> MSRRPTLRLGLDRDVYNIVLNLEQQGTDENGKRPRLTVDYVYDTIKRSNSSLARQKKRMLEDSIERVLAVRKEQAKAEEETDSDDLIEAQERERERQKAAQAQRDANLLNR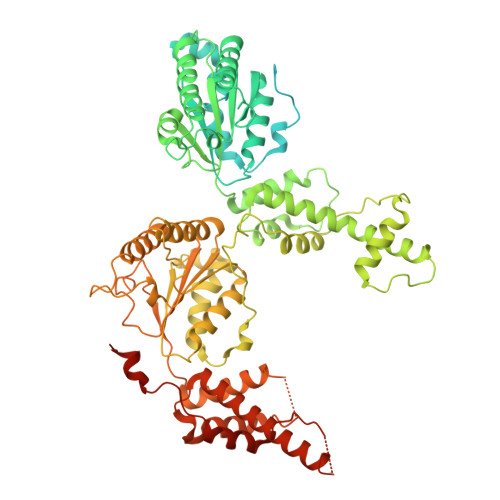QIAKSWGFASSPGAKAADGEKGTDTGSIATPAPATPAVAENMAADTPTTSTGPVLPASSTDRQPNGEPRPKKRKAAPKEIDRTPPTKVSILDIAGVDDTLQRLLKEVWFPLRGGEACEKMGYRYDNGVLLHGPSGCGKTTLAHAIAGSIGVAFIPVSAPSVIGGTSGESEKNIRDVFDEAIRLAPCLIFLDEIDAIAGRRESANKGMESRIVAEIMNGMDRIRQNTPLGKNVVVLAATNRPEFLDPAIRRRFSVEIDMGMPSERAREQILRSLTRDLSLADDINFKELAKMTPGYVGSDLQYVVKAAVSESFQANIDSLLAQARAKHPADHLANVSQPQRDWLLLEAHRDEEVSWPSTKITMEQFRKAVSLVQPASKREGFSTIPDTTWSHVGALEDVRKKLEMSIIGPIKNPELFTRVGIKPAAGILLWGPPGCGKTLVAKAVANESKANFISIKGPELLNKYVGESERAVRQLFSRAKSSAPCILFFDQMDALVPRRDDSLSDASARVVNTLLTELDGVGDRSGIYVIGATNRPDMIDEAIRRPGRLGTSIYVGLPSAEDRVKILKTLYRNTVKAPKKREGTNGEDVDMTDAAAEQQHQGTTDADLEKVALDLRCTGFSGADLGNLMQAAAQACLERVYTQRQQKRKEGGSVAEEEEIEPVITMEDWEKALNEVKPSVKDPEKYMHSGFAAALEHHHHHH> K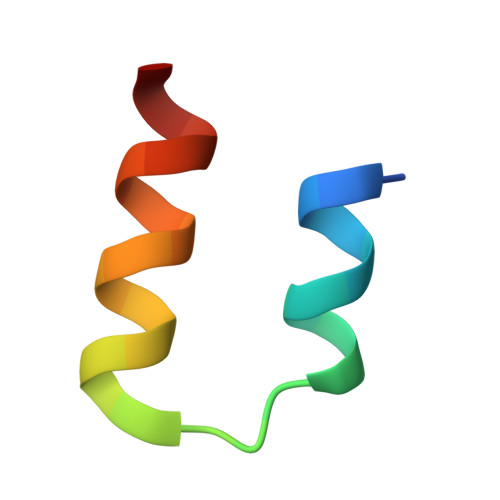HKILHRLLQDSSSPVDLAKLTAEATGK As the first reported host of “non-pathogenic-derived” pili, Lactobacillus rhamnosus GG is a gut-adapted commensal lactic acid bacterium (LAB) and one of many clinically investigated probiotic strains for human use in the prevention and treatment of certain gastric ailments. As with other Gram-positive bacteria, sortase-dependent piliation in L. rhamnosus GG (called SpaCBA) is assembled from the ~30 kDa SpaA (backbone), ~20 kDa SpaB (basal), and ~90 kDa SpaC (tip-located) pilins. Two immunoglobulin (Ig)-like subdomains comprise GG-SpaA, each having the conserved residues of a canonical E-box motif and internal isopeptide bonds formed between either lysine and asparagine or lysine and aspartate residues. Our findings show that the GG-SpaA structure has certain features in common with other pathogen-derived pilin-proteins, such as the Ig-like CnaB-type folds and the presence of internal isopeptide bonds6940.

Included in these experiments was also a related third mutant, in which the aspartate that forms the isopeptide bond in the C-domain was substituted with an asparagine (i.e., D295N), the residue that is normally found in Gram-positive backbone pilins. D295N-substituted GG-SpaA crystallizes in the same space group as the full-length WT protein and the E139A and E269A mutants, though with different cell dimensions. Six molecules in the asymmetric unit were visible, where the N-domain of one molecule is facing the C-domain of an adjacent molecule as in full-length WT. The overall topology of the D295N crystal structure is similar to that of WT GG-SpaA (RMSD of 0.8 Å), with maximum structural deviations found at the AB loop. Significantly, the electron density between Lys184 and the substituted Asn295 clearly supports the formation of an isopeptide bond. Here, a protein band (~30 kDa) representing WT and D295N-mutated GG-SpaA was seen to be present throughout the 24 hours of trypsinization, although trace amounts of a smaller ~16 kDa-sized band began to be detected following 3 hours of incubation, with the levels then continuing to increase over time. The results suggest that the resistance to proteolysis apparently displayed by the WT and D295N can be correlated more with isopeptide bond in C-domain than that in the N-domain of GG-SpaA. Here, a first and second Tm for both the WT and D295N proteins was observed at around 52 and 66 °C, respectively.

>MGRDPNSTNDTTTQNVVLTKYGFDKDVTAIDRATDQIWTGDGAKPLQGVDFTIYNVTANYWASPKDYKGSFDSAPVAATGTTNDKGQLTQALPIQSKDASGKTRAAVYLFHETNPRAGYNTSADFWLTLPAKAAADGNVYVYPKNVQKTTYERTFVKKDAETKEVLEGAGFKISNSDGKFLKLTDKDGQSVSIGEGFIDVLANNYRLTWVAESDATVFTSDKSGKFGLNGFADNTTTYTAVETNVPDGYDAAANTDFKADNSSSDILNAPSGILPLEHHHHHH[6x]>TSNFFCGEPIDYRGITAHRLVGAEPRPPVSGTRYAKVPGVPDEYKTGYRPANLGRSDPDSDKSLMNIAVKNLQVYQQEPKLDKVDEFIERAAADVLGYLRFLTKGERQANLNFKAAFNTLDLSTSCGPFVPGKKIDHVKDGVMDQVLAKHLYKCWSVANSGKALHHIYACGLKDELRPLDKVKEGKKRLLWGCDVGVAVCAAAVFHNICYKLKMVARFGPIAVGVDMTSRDVDVIINNLTSKASDFLCLDYSKWDSTMSPCVVRLAIDIL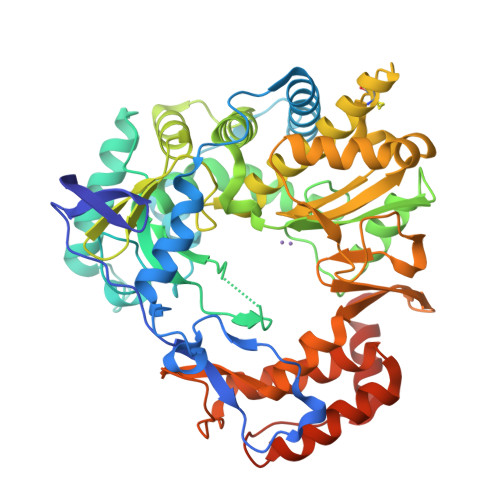ADCCEQTELTKSVVLTLKSHPMTILDAMIVQTKRGLPSGMPFTSVINSICHWLLWSAAVYKSCAEIGLHCSNLYEDAPFYTYGDDGVYAMTPMMVSLLPAIIENLRDYGLSPTAADKTEFIDVCPLNKISFLKRTFELTDIGWVSKLDKSSILRQLEWSKTTSRHMVIEETYDLAKEERGVQLEELQVAAAAHGQEFFNFVCRELERQQAYTQFSVYSYDAARKILADRKRVVSVVPDDEFVNVME[2x]> GGGRVDHVFYQKFKSMALQELGTNYLSISYVPSLSKFLSKNLRSMKNCIVFFDKVEHIHQYAGIDRAVSETLSLVDINVVIIEMNDYLMKEGIQSSKSKECIESMGQASYSGQLDFEASEKPSNHTSDLMMMVMRKINN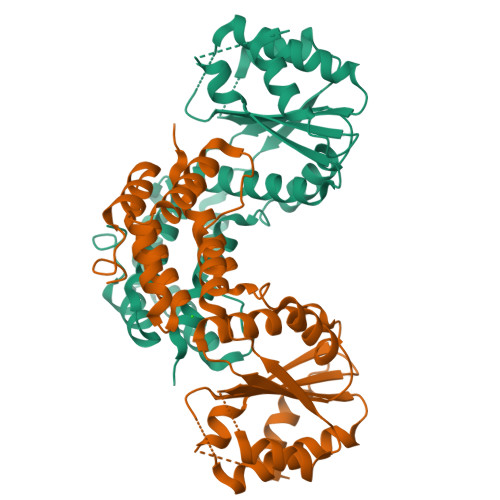DESIDHIVYFKFEQLDKLSTSTIIEPSKLTEFINVLSVLEKSNNIAFKVLIYSNNVSISSLLSTSLKKKLNTKYTVFEMPILTCAQEQEYLKKMIKFTFDSGSKLLQSYNSLVTCQLNNKESNLAIFFEFLKVFPHPFTYLFNAYTEIIVQSRTFDELLDKIRNRLTIKNYPHSAYNFKK We recently reported a flavin‐trafficking protein (Ftp) in the syphilis spirochete Treponema pallidum (Ftp_Tp) as the first bacterial metal‐dependent FAD pyrophosphatase that hydrolyzes FAD into AMP and FMN in the periplasm. Orthologs of Ftp_Tp in other bacteria (formerly ApbE) appear to lack this hydrolytic activity; rather, they flavinylate the redox subunit, NqrC, via their metal‐dependent FMN transferase activity. In the current study, we identified a bimetal center in the crystal structure of Escherichia coli Ftp (Ftp_Ec) and show via mutagenesis that a single amino acid substitution converts it from an FAD‐binding protein to a Mg2+‐dependent FAD pyrophosphatase (Ftp_Tp‐like). A high‐resolution structure of the Ftp‐mediated flavinylated protein of Shewanella oneidensis NqrC identified an essential lysine in phosphoester‐threonyl‐FMN bond formation in the posttranslationally modified flavoproteins.

John Wiley & Sons, LtdAs the Ftp_EcY60N protein variant displays FAD pyrophosphatase activity that is inhibited by ADP, we obtained a crystal structure of the ADP complex with two metals bound. This structure provides the best model to date of the bimetal coordination of the ADP portion of an FAD substrate to this subclass of FMN transferases. In contrast to the apo structures, there are only two monomers in the asymmetric unit, and the r.m.s.d. of the monomers is 0.4 Å for 289 Cα carbons. The metal ion in site 1 in both monomers is no longer coordinated to a carboxylate oxygen atom from the side chain of D283, and thus has a coordination number of 6. Refinement of the metals as Ca2+ ions resulted in large negative electron density peaks that disappeared when modeled and refined as Mg2+ ions. Unlike the Ftp_Tp ADP‐inhibited structure, the α‐phosphate oxygens of the ADP do not coordinate to the metal ion in site 1. Coordinated to a second Mg2+ ion are α‐ and β‐phosphate oxygens of the ADP, as well as the side chain of E169. The side chain of R240 also coordinates to the β‐phosphate of the ADP. The distance between metal sites in this structure is over 6 Å, approximately twice the distance observed in the various Ftp_Tp inhibitor and substrate complexes, and we observed no metal‐coordinated water that can effectively bridge between the bimetal sites. Despite the presence of a Ca2+ ion in metal site 1 in the apo enzyme, the inhibited Ftp_EcY60N protein variant enzyme contains a bimetal Mg2+ center.

>[2x]MDQKPQPAKTHATEVTVLEGKTMGTFWRASIPGIDAKRSAELKEKIQTQLDADDQLLSTNKKDSALMRFNDSQSLSPWPVSEAMADIVTTSLRIGAKTDGAMDITVGPLVNLWGFGPEQQPVQIPSQEQIDAMKAKTGLQHLTVINQSHQQYLQKDLPDLYVDLSTVGEGYAADHLARLMEQEGISRYLVSVGGALNSRGMNGEGLPWRVAIQKPTDKENAVQAVVDINGHGISTSGSYRNYYELDGKRLSHVIDPQTGRPIEHNLVSVTVIAPTALEADAWDTGLMVLGPEKAKEVVRREGLAVYMITKEGDSFKTWMSPQFKSFLVSEKNLEHHHHHH>[2x]MISMKPRYKPDWESLREHTVPKWFDK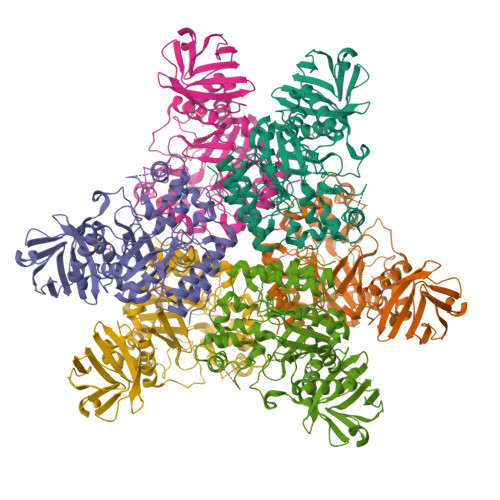AKFGIFIHWGIYSVPGWATPTGELGKVPMDAWFFQNPYAEWYENSLRIKESPTWEYHVKTYGENFEYEKFADLFTAEKWDPQEWADLFKKAGAKYVIPTTKHHDGFCLWGTKYTDFNSVKRGPKRDLVGDLAKAVREAGLRFGVYYSGGLDWRFTTEPIRYPEDLSYIRPNTYEYADYAYKQVMELVDLYLPDVLWNDMGWPEKGKEDLKYLFAYYYNKHPEGSVNDRWGVPHWDFKTAEYHVNYPGDLPGYKWEFTRGIGLSFGYNRNEGPEHMLSVEQLVYTLVDVVSKGGNLLLNVGPKGDGTIPDLQKERLLGLGEWLRKYGDAIYGTSVWERCCAKTEDGTEIRFTRKCNRIFVIFLGIPTGEKIVIEDLNLSAGTVRHFLTGERLSFKNVGKNLEITVPKKLLETDSITLVLEAVEE>MEFMSAPANAVAADDATAIALKYNQDATKSERVAAARPGLPPEEQHCANCQFMQAD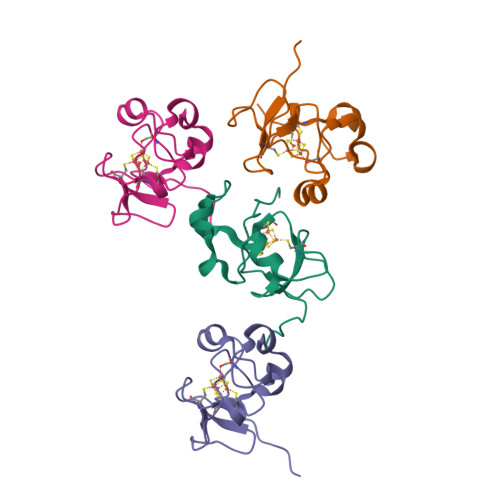AAGATDEWKGCQLFPGKLINVNGWSASWTLKAG[4x]>SQIIRCKAAVAWEAGKPLVIEEVEVAPPQKHEVRIKILFTSLCHTDVYFWEAKGQTPLFPRIFGHEAGGIVESVGEGVTDLQPGDHVLPIFTGECGECRHCHSEESNMCDLLRINTERGGMIHDGESRFSINGKPIYHFLGTSTFSEYTVVHSGQVAKINPDAPLDKVCIVSCGLSTGLGATLNVAKPKKGQSVAIFGLGAVGLGAAEGARIAGASRIIGVDFNSKRFDQAKEFGVTECVNPKDHDKPIQQVIAEMTDGGVDRSVECTGSVQAMIQAFECVHDGWGVAVLVGVPSKDDAFKTHPMNFLNERTLKGTFFGNYKP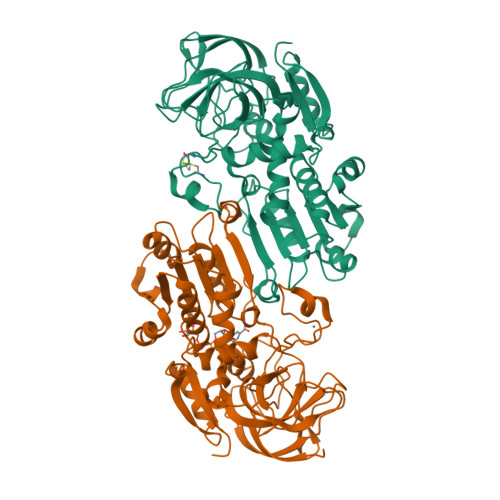KTDIPGVVEKYMNKELELEKFITHTVPFSEINKAFDYMLKGESIRCIITMGA[2x]>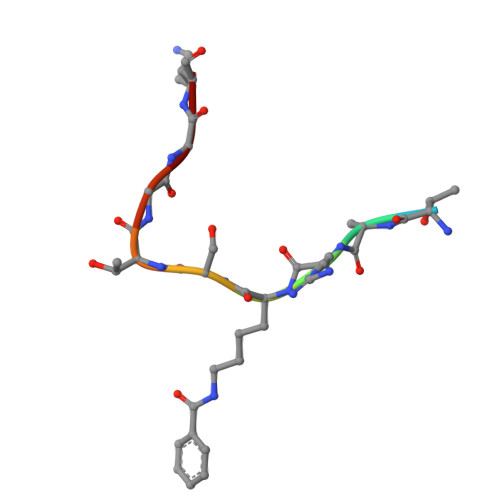 QTARKSTGGK>MADPLTPAISDRICKHMNEDHASAIALYAQVFGQQTDVTMAQMQAIDPTGMDLVVESEGGSKTIRIEFEQPLKDSEDAHQVLIAMAKQARSVGKNSAENLYFQ[4x]

Using a phylogenomics-based approach and complementary structural techniques, we identify a family of dimeric hemoproteins comprising a domain of unknown function DUF2470. The heme iron is axially coordinated by two zinc-bound histidine residues, forming a distinct two-fold symmetric zinc-histidine-iron-histidine-zinc site. Together with structure-guided in vitro and in vivo experiments, we further demonstrate the existence of a functional link between heme binding by Dri1 (Domain related to iron 1, formerly ssr1698) and post-translational regulation of succinate dehydrogenase in the cyanobacterium Synechocystis, suggesting an iron-dependent regulatory link between photosynthesis and respiration. Given the ubiquity of proteins containing homologous domains and connections to heme metabolism across eukaryotes and prokaryotes, we propose that DRI (Domain Related to Iron; formerly DUF2470) functions at the molecular level as a heme-dependent regulatory domain. We heterologously expressed and purified the recombinant protein encoded by the Synechocystis gene dri1 (formerly known as ssr1698) and tested the heme-binding ability of this small, soluble protein (96 amino acids, 10 kDa).

The heme-bound form is a homodimer consisting of two monomeric chains running in the same N-C direction. Although the homodimer maintains the same monomeric fold per chain, a two-fold-symmetric zinc-mirror site binds a single heme cofactor (Supplementary Fig. 3 for electron density maps). The heme iron is axially ligated at the interface of the dimer by His79 (Nε2; 2.04–2.13 Å) from each monomer. His79 (Nδ1; 2.11–2.14 Å) is in turn bound to a zinc ion that is additionally ligated by His16, His21, and Glu76. The heme propionate groups form a salt bridge with an Arg90 side chain from each monomer. In turn, two zinc-bound histidine residues, one from each monomeric chain, coordinate to the iron center of a single heme cofactor. These zinc ions may help catalyze the formation of the imidazole-iron bonds by increasing the basicity of the histidine Nε2 atoms in a charge-relay fashion and/or play a structural role responsible for the precise positioning of heme between the two monomers. However, we report here a protein possessing a two-fold symmetric zinc-histidine-heme iron-histidine-zinc coordination center at the interface of a homodimer. SEC-SAXS shows that heme binding pushes the system primarily into the dimer state and no higher-order oligomers or unreacted monomers are present. Based on the structure of Dri1, we propose that heme binding leads to a Dri1 homodimer that can no longer bind to SdhB1.>GMGVNMRAETESRIFSVDEYVRPSNGEPIRSVVLETNDSVVVVWHAHPGQEIASHVHPHGQDTWTVISGEAEYHQGNGIVTHLKAGDIAIAKPGQVHGAMNSGPEPFIFVSVVAPGNA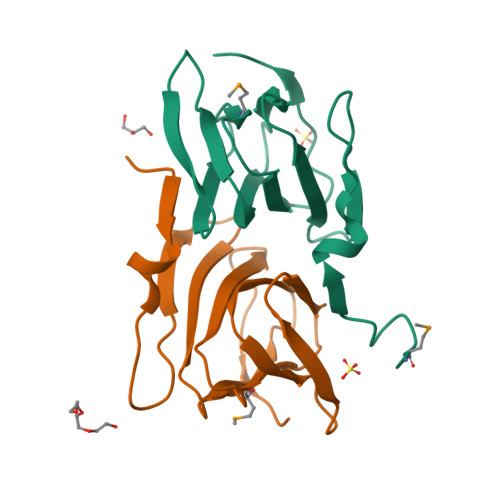GFALAEK[2x]> MTGIPTVTARPWTQRPRAENSTTNPTYFFTFGDSYSQTGFSASGTQPSASNPMGNPDLGIGTTTNGPNWIGYLTTTENASLVLSYNLAAGGATIDNALVPFYPGDLASQFRLFEDVYADKPASAPWSAEDAVFGVWIGINDIGNAYYSTDAETYTPKLISRLESLVEEVYKNGGRKFLFLNV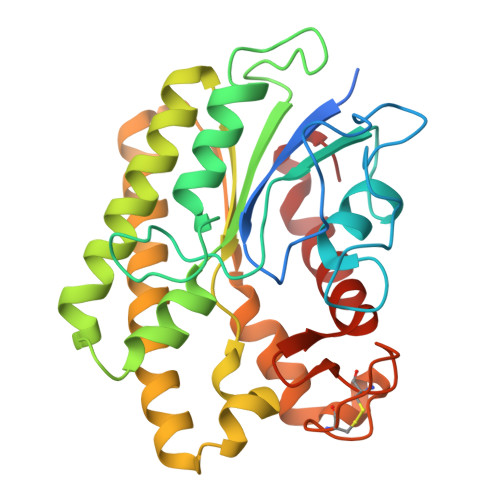PPTSRSPLFLEQGEEVVKQHAEYLSVYNENLEGMVDDFTKKKGDVTTVLYDSWSFMTKILDDPTAYGFPDATCINDDGTSCIWWDNYHPGMKYHLLQAEDMKPKLRKLGGW> RSVYELDCIPLWGTVSIQGNRSEMEDAFAVSPHFLKLPIKMLMGDHEGMSPSLTHLTGHFFGVYDGHGGHKVADYCRDRLHFALAEEIERIKDELCKRNTGEGRQVQWDKVFTSCFLTVDGEIEGKIGRAVVGSSDKVLEAVASETVGSTAVVALVCSSHIVVSNCGDSRAVLFRGKEAMPLSVD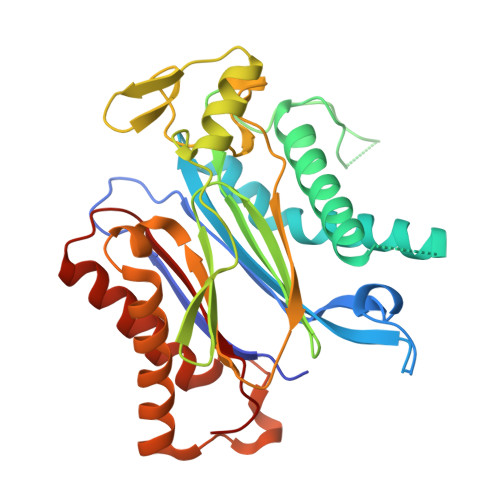HKPDREDEYARIENAGGKVIQWQGARVFGVLAMSRSIGDRYLKPYVIPEPEVTFMPRSREDECLILASDGLWDVMNNQEVCEIARRRILMWHKKNGAPPLAERGKGIDPACQAAADYLSMLALQKGSKDNISIIVIDLKAQR>GSMEEFVKVRKKDLERLTTEVMQIRDFLPRILNGELLESFQKLKMVEKNLERKEQELEQLIMD[2x];>[2x]GSMRMQDATDTVRGLV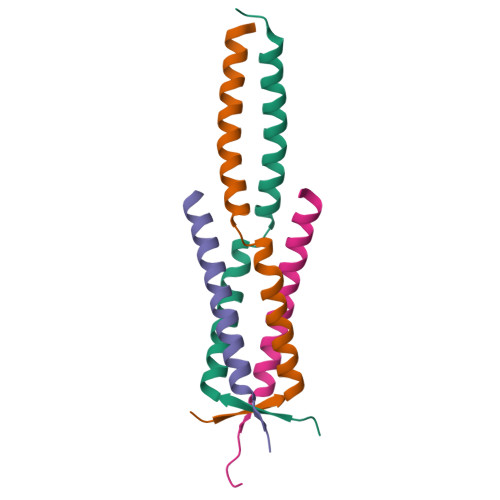VELSGLNRLIMSTHRDLEAFKR> MFKSLALVALATISPSALCAPITSRDIPFGQVITTCTTPNTVALTFDDGPSSYTPQLLDLLSEYKVRATFFVLGEASQSNPQIIQRIRQEGHQVGSHTYDHTSLPTLSYDQIVQEMTSLESVLQSTMGDIPTYMRPPYFDVNDLTLQVMSDLGYHVVTASIDTKDYNHNSPDLISQSYDKFVTELNNGGNLCLAHDTKEQTVVTLAKMMLDETKSRGLTVTTVGDCLGDPEASWYRSSR

Chitin deacetylases (CDAs) are found in many different organisms ranging from marine bacteria to fungi and insects. These enzymes catalyze the removal of acetyl groups from chitinous substrates generating various chitosans, linear copolymers consisting of N-acetylglucosamine (GlcNAc) and glucosamine. All CE4 enzymes are metalloenzymes that share a similar fold and five conserved motifs forming the substrate-binding site. This binding site is comprised of several subsites, with subsite 0 binding the sugar unit being deacetylated and the minus and plus subsites accommodating the units toward the nonreducing and reducing ends, respectively.

In this study, we analyzed AngCDA, an Aspergillus niger CDA that is strongly expressed in the mutant scl-2, which in contrast to the wildtype forms sclerotia, a survival structure for harsh environmental conditions and a prerequisite for sexual reproduction. To further elucidate the substrate-binding site, the X-ray crystal structure of AngCDA was determined at a resolution of 1.81 Å. The enzyme crystallized in the space group P432 with one monomer per asymmetric unit. AngCDA adopts a distorted (α/β)8 fold, as typically found in CE4 enzymes. The conserved Asp–His–His triad (Nε2-H97, Nε2-H101, and Oδ1-D48 atoms) plus a malonate ion (O6 and O7 atoms) from the crystallization solution and a water molecule coordinate a zinc(II) ion to form an octahedral coordination geometry with a metal–ligand distance of 2.2 Å. The malonate ion is found at the expected subsite 0, where the acetyl group of the chitinous substrate is normally placed and hydrolyzed. All five conserved motifs can be found in AngCDA, with motif 1 harboring the catalytic base (D47) and the metal-binding aspartate (D48) and motif 2 containing both metal-binding histidines (H97 and H101). Motif 3 includes an arginine (R135), which properly orients the catalytic aspartate (D47) and a tyrosine (Y138) forming a hydrogen bond with the acetyl oxygen at subsite 0. Motif 4 contains an aspartate (D165) that enables the protonation of the catalytic histidine (H195), and motif 5 contains a leucine (L193) forming one side of the hydrophobic pocket for the acetamido's methyl group at subsite 0 and the catalytic acid (H195). We found that Aspergillus niger CDA strongly prefers a GlcNAc sugar unit at its −1 subsite and shows a weak GlcNAc preference at the other noncatalytic subsites, which was apparent both when deacetylating and N-acetylating oligomeric substrates.> MSQSNRELVVDFLSYKLSQKGYSWSQFSDVEENRTEAPEGTESEAVKQALREAGDEFELRYRRAFSDLTSQLHITPGTAYQSFEQVVNELFRDGVNWGRIVAFFSFGGALCVESVDKEMQVLVSRIAAWMATYLNDHLEPWIQENGGWDTFVELYGNNAAAESRKGQER

The Bcl-2 family of proteins is a key apoptotic regulator in response to a wide variety of stimuli perturbing cellular homeostasis. The antiapoptotic Bcl-2 proteins interact with the proapoptotic Bcl-2 family members and prevent the formation of an oligomeric pore in the mitochondrial outer membrane (MOM). In contrast, Bcl-xL primarily resides in the mitochondrial outer membrane with the C-terminal helix embedded at the mitochondrial membrane and induces small, transient alterations of the membrane permeability without affecting consequences for the MOMP12. Apart from modulating MOMP directly, the Bcl-2 family proteins and Bcl-xL in particular regulate the calcium homeostasis through interactions with Voltage Gated Anion Channel (VDAC), a MOM protein.

To delineate the poorly understood structural transition steps between water-soluble and membrane-bound conformations of Bcl-xL and ultimately the molecular mechanism of Bcl-xL, we determined the X-ray crystal structure of Bcl-xL in the presence of the detergent n-Octyl β-D-Maltoside (OM). As the full-length Bcl-xL (Bcl-xLFL) and the C-terminal and loop-truncated Bcl-xL (Bcl-xL∆L∆CT) show similar structural folds and BH3 peptide binding profiles, as assessed by two-dimensional (2D) 1H-15N TROSY-HSQC and HSQC spectra, we used the soluble Bcl-xL∆L∆CT (referred to as Bcl-xL hereafter) for our structural studies. n-Octyl β-D-Maltoside (OM) was the detergent used to study the oligomerization properties of Bcl-xL. In the dimeric conformation helices α6-α8 of one Bcl-xL molecule are reciprocally exchanged with α6′-α8′ of the other, retaining the hydrophobic binding pocket exposed to solvent. The helices α5 and α6 in the water-soluble structure fuse into a single long helix, which interacts with the equivalent helix from the neighboring unit oriented in an anti-parallel direction. The dimer interface (monomer-monomer) area, calculated by the software PISA23, was ~3215 Å2 made up of a total of 79 residues. In the structure presented here, the crystal symmetry generated a hexameric assembly, a trimer of dimers, which was not observed in the previously reported pH induced dimer21. But the dimer-dimer interface is weak indicating that the hexamer could be a transient oligomer or just an effect of crystal packing. Similarly a major conformational change is observed in the α5-α6 loop, which converts to an alpha helix in the dimeric form. The solution Rg and Dmax values match well with the dimeric crystal structure Rg value of 24.5 Å and the Dmax of 79.6 Å. The mutations E158P and M159P arrested the OM induced dimer formation of Bcl-xL, indicating that the α5-α6 loop region is critical for Bcl-xL dimer formation.>MTATLAAPSKTRRVVFPFTAIVGQDEMKLALLLNVIDPKIGGVMIMGDRGTGKSTTIRALADLLPEIEVVANDPFNSSPSDPEMMSEEVRIRVDSQEPLSIVKKKVTMVDLPLGATEDRVCGTIDIEKALSEGVKAFEPGLLAKANRGILYVDEVNLLDD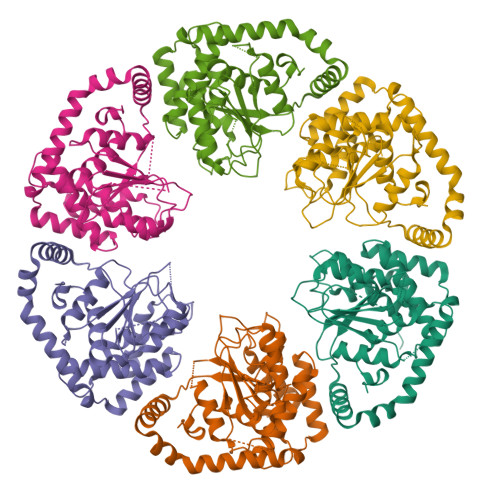HLVDVLLDSAAGGWNTVEREGISIRHPARFVLVGSGNPEEGELRPQLLDRFGMHAEIRTVREPELRVKIVEQRTEFDQNPHPFCDQYQTEQEALQAKIVNAQNLLPQVTIDYDYRVKVSEVCAELDVDGLRGDIVTNRAAKALAAFEGRTEVTVDDISRVIVLCLRHRLRKDPLESIDSGSKVEKVFKRVFGVVDEALEHHHHHH[6x]> E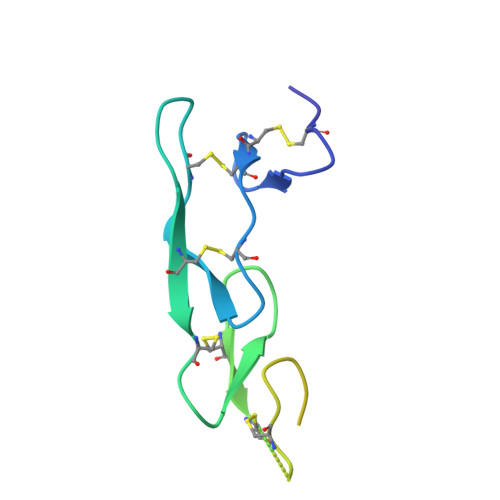ICKPEEVQLGDQCCPPCKQGYRVTGQCTQYTSTTCTLCPSGTYVSGLYQCTQCTECQDTEVTIRNCTSTQNTVCASKQYTSFSVPGVQHHKQRQSHTAHVTVKQGKSGRHTHHHHHH> SNAIGTDSKFGVDLSTQAAKSYNTKTIVAAKRGTIYDRNGNVLAEDSTSYSIYAIVSTSYVSPTREKLYVQESQFDKVADILKDKLGIKKSYTLAQLRTKGAYQVSFGLKGKGITYSVKEDLEKTFKDAGIKGMAFEATTSRMYPNGTFASEFLGRAEPIENKKDGSYSLIGQTGLERSLNSLLTGTDGEAIYEKDKDGNTLLGTETITKEAIDGKNIYTTLSAPLQTFLETQMDTFMEQTKGINASATVVNAKTGEILATTQRPTYNSDTLEGQAKKGYDWVNRLYEAQYEPGSTMKVMLLSAAINNGSFNPNATYSNANGIKVGDVEINDWSINEGISKGRTMSFAQGFSYSSNVGMTMLEQAMGDKVWSNYLSLYKFGIPTRFGMVGESSGIVSQNSVNIAQSSFGQGISVTQVQMLRAFTAISNNGIMLEPQFIKQVADTNKGTVRTAKKEVIGKPVSKQAASETRNYMISVGTDPEFGTLYNKSEGSPIIQVGNNDVTVKSGTAQVPDEKTGTYKVGTNETLNSVVAMVPSEDPEYIMYVTVQEPKTWNNNFFATVVNPVLEEAMSMGATLDTSVSEGSGKTEETSYQTGDIIGKTPGETANTLRQNLVHPIVLGVGNKIEKVSVDAKENIKANEQILIMTNEFTELPDMYGWTKKNVETFAKWK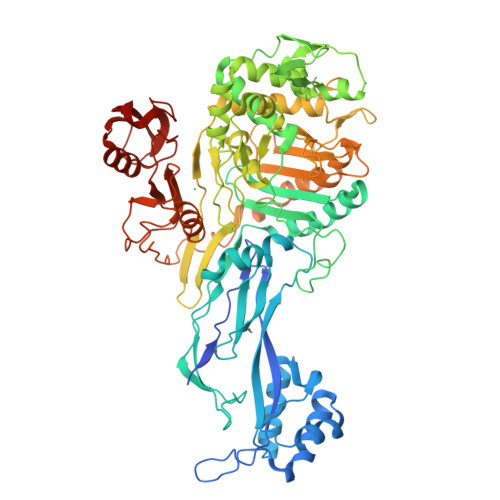GIKITYKGGKSGTVTKQSVAAGEALSKTKKITITLGD>[4x]MIIFSGGTGTPKLLDGLKEILPEEELTVVVNTAEDLWVSGNLISPDLDTVLYLFSDQIDRKRWWGIENDTFGTYERMKELGIEEGLKLGDRDRATHIIRSNIIRDGASLTDSTVKLSSLFGIKANILPMSDDPVSTYIETAEGIMHFQDFWIGKRGEPDVRGVDIRGVSEASISPKVLEA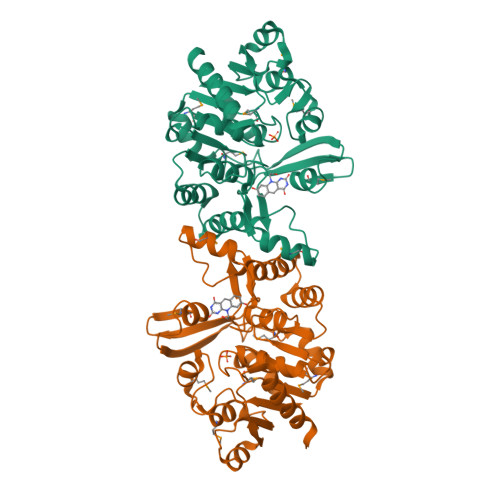FEKEENILIGPSNPITSIGPIISLPGMRELLKKKKVVAVSPIIGNAPVSGPAGKLMPACGIEVSSMGVAEYYQDFLDVFVFDERDRADEFAFERLGCHASRADTLMTSTEKSKELAEIVVQAFLEHHHHHH> MGHHHHHHGTENLYFQGSAATMAAQSLLSIPVEYRSQVWCRANLPYPPAPQLPIPAVVDILTKASQALPQISFSWTLIDQPPDGSLFLVWQAPTLPSPPDGMHFMSNERFFNMDVAGKVLEIHEAKHGFYPLSETRTMHVRCRYRLLGVGFDNFWLVHYFQGSETDSIPANISVAKPPHLRRYPLPDVKTSPF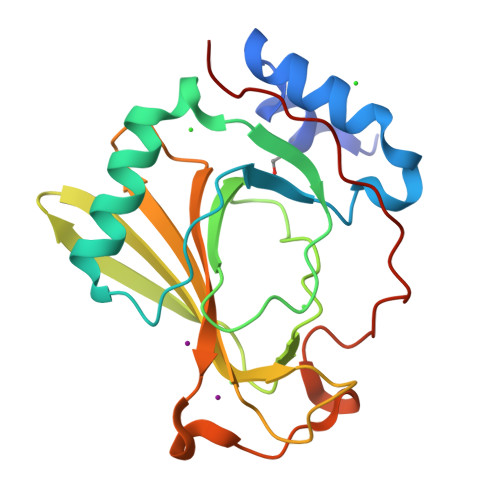LLQE> MPEVVGSYFQSNAMTGPHAAGGSNHRTARLVAIIAGLLGTLMAIATPLLPVEQTTAELNWPQNGVWQSVDAPLIGYVATDLTVTVPCQAAAGLVGPENRNRSVLLSTVPKQAPKAIDRGLLIERINNDLTVIVRNTPVVSAPLEQVLSPDCRYLTFTAHADKVTGEFVGLTQGPDDDDPGEAVRGERSGYDFRPQIVGVFTDLSG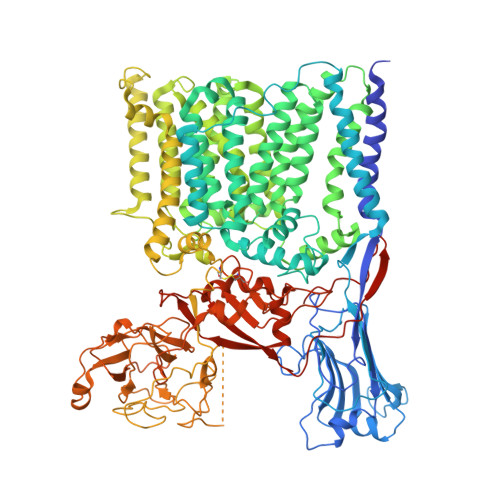PAPEGLQLSATIDTRYSTSPTLLKLLAMIVGVAMTVIALGALHVLDCADGRRHKRFLPSRWWSMTPLDGLVSAMLVWWHFVGANTADDGYILTMARVSEHAGYMANYYRWFGTPESPFGWYYDLLALWAHVSTASVWMRFPTLLMGLACWWVISREVIPRLGAAAKHSRAAAWTAAGLFLAFWLPLNNGLRPEPIIALGILLTWCSVERGVATSRLLPVAVAIIIGALTLFSGPTGIAAVGALLVAIGPLKTIVAAHVSRFGYWALLAPIAAAGTVTIFLIFRDQTLAAELQASSFKSAVGPSLAWFDEHIRYSRLFTTSPDGSVARRFAVLTLLLALAVSIAMTLRKGRIPGTALGPSRRIIGITIISFLAMMFTPTKWTHHFGVFAGLAGCLGALAAVAVTTTAMKSRRNRTVFGAAVLFVTALSFATVNGWWYVSNFGVPWSNSFPEFKFGFTTMLLGLSVLALLVAAWFHFSGRDVSPDRPQRRWQRLLVAPLAVATWALVIFEVVSLTLGMINQYPAWSVGRSNLNALTGKTCGLANDVLVEQNANAGMLTPIGEPAGQALGAVTSLGFGPNGIPSDVSADPVMEQPGTDNFADSDSGVVTGTEVGTEGGTTAAAGINGSRARLPYGLNPATTPVLGSWRSGTQQPAVLRSAWYRLPDRDQAGPLLVVSAAGRFDQGEVEVQWATDEQAAANEPGGSITFGDVGAAPAWRNLRAPLSSIPPEATQIRLVASDDDLAPQHWIALTPPRIPELRTLQEVVGSSDPVMLDWLVGLAFPCQRPFDHRYGVVEVPKWRILPDRFGAEANSPVMDYLGGGPLGITELLLRPSSVPTYLKDDWYRDWGSLQRLTPWYPDAQPARLDLGTATRSGWWSPAPLRLSHLGGIKAFLEVLFQGPHHHHHHHHHH HIV-1 reverse transcriptase (RT) copies the viral ~10-kilobase ssRNA genome to a dsDNA in a multistep process. For the DNA synthesis, RT binds an eighteen-base-pair stretch of a duplex substrate with the primer 3′-end nucleotide occupying the priming site (P site). A dNTP complementing the first template overhang binds the N site and the nucleotide part is catalytically incorporated by RT at the 3′-end of the primer with the release of pyrophosphate. Following each nucleotide incorporation, the DNA is translocated from N to P site to accommodate the next dNTP.

Fragment 048 is smaller in size and contains two rings—a cyclopropyl and a pyrazole. The cyclopropyl group is the only chemical moiety common to both fragments 048 and 166, and the cyclopropyl group occupies a common area of P-pocket in both structures, despite that two fragments fill different parts of the pocket. The cyclopropyl ring is positioned over the YMDD motif in the pocket, and like 166, fragment 048 binding knocks out the active site Mg2+ ion. The 4-bromopyrazole ring interacts with the residues Y115 and Q151 and points toward the dNTP-binding site (or N site). The 4-bromopyrazole moiety is stacked against Y115 sidechain and the bromine atom interacts with the Q151 sidechain. The pocket rearrangement is less extensive for accommodating 048 compared with 166, which indicates elasticity of this transient P-pocket. The deoxyribose ring of the primer 3′-end nucleotide and the YMDD motif each shifts by ~1.3 Å for binding 048 when compared with the apo structure. A superposition of 166- and 048-bound RT/DNA structures suggests the potential for P-pocket to accommodating different chemical moieties at different parts. There exist multiple opportunities to design compounds with pocket-specific interactions such as pseudo A:T or G:C base-pairing and extension to reach active site, primer grip, and key residues such as Y115 and M151 that are involved in dNTP binding; binding of fragment 048 indicates the potential for acquiring interactions with Y115 and M151.

>MVPISPIETVPVKLKPGMDGPKVKQWPLTEEKIKALVEICTEMEKEGKISKIGPENPYNTPVFACKKKDSTKWRKLVDFRELNKRTQDFWEVQLGIPHPAGLKKKKSVTVLDVGDAYFSVPLDEDFRKYTAFTIPSINNETPGIRYQYNVLPQGWKGSPAIFQSSMTKILEPFKKQNPDIVIYQYMDDLYVGSDLEIGQHRTKIEELRQHLLRWGLTTPDKKHQKEPPFLWMGYELHPDKWTVQPIVLPEKDSWTVNDIQKLVGKLNWASQIYPGIKVRQLSKLLRGTKALTEVIPLTEEAELELAENREILKEPVHGVYYDPSKDLIAEIQKQGQGQWTYQIYQEPFKNLKTGKYARMRGAHTNDVKQLTEAVQKITTESIVIWGKTPKFKLPIQKETWETWWTEYWQATWIPEWEFVNTPPLVKLWYQLEKEPIVGAETFYVDGAANRETKLGKAGYVTNKGRQKVVPLTNTTNQKTELQAIYLALQDSGLEVNIVTDSQYALGIIQAQPDKSESELVNQIIEQLIKKEKVYLAWVPAHKGIGGNEQVDKLVSA[2x];>MAHHHHHHALEVLFQGPISPIETVPVKLKPGMDGPKVKQWPLTEEKIKALVEICTEMEKEGKISKIGPENPYNTPVFAIKKKDSTKWRKLVDFRELNKRTQDFWEVQLGIPHPAGLKKKKSVTVLDVGDAYFSVPLDEDFRKYTAFTIPSINNETPGIRYQYNVLPQGWKGSPAIFQSSMTKILEPFKKQNPDIVIYQYMDDLYVGSDLEIGQHRTKIEELRQHLLRWGLTTPDKKHQKEPPFLWMGYELHPDKWTVQPIVLPEKDSWTVNDIQKLVGKLNWASQIYPGIKVRQLSKLLRGTKALTEVIPLTEEAELELAENREILKEPVHGVYYDPSKDLIAEIQKQGQGQWTYQIYQEPFKNLKTGKYARMRGAHTNDVKQLTEAVQKITTESIVIWGKTPKFKLPIQKETWETWWTEYWQATWIPEWEFVNTPPLVKLWYQ[2x]> MATRADEDGDTPLHIAVVQGNLPAVHRLVNLFQQGGRELDIYNNLRQTPLHLAVITTLPSVVRLLVTAGASPMALDRHGQTAAHLACEHRSPTCLRALLDSAAPGTLDLEARNYDGLTALHVAVNTECQETVQLLLERGADIDAVDIKSGRSPLI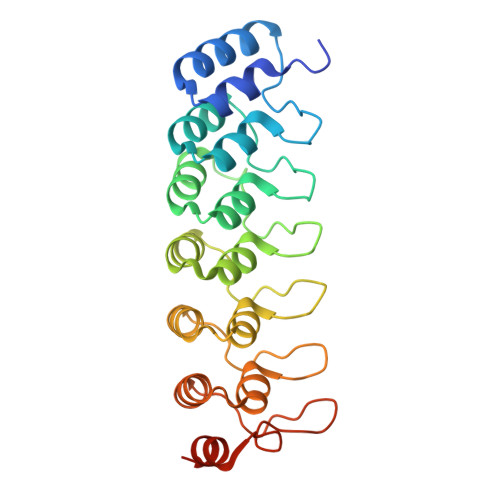HAVENNSLSMVQLLLQHGANVNAQMYSGSSALHSASGRGLLPLVRTLVRSGADSSLKNCHNDTPLMVARSRRVIDILRGKATRPAS>QGMDFTLNQEMLMTDTKSGALFYQEEEALSGVRKIANKVMHDVELVFGYQPEATKDRDMLSRHAVLYGTVGHSPLLDELNAAALIDLTEIAGKREVFLFQVVDQPIQGVEKALVIAGSDKRGTIYGLFHLSEKLGVSPLVDWSGVLPARKESFSLKGDYKYVSKEPSVKYRGFFINDEWPAFGNWSAKNFGGFNAEMYDHVFELLLRLKGNYLWPAMWSARFNDDGPGLANVELADEYGVIMGASHHEPCLRYGEEYKYLRGPDSIYGDAWNFITNREGITKFWEDGLKRTGHFENIITIGMRGEADTKIMGEDATLEDNINLLRDVIQTQNKLIKEHVNPNLKEVPRMLALYKEVEPFFYGDENTPGLINSEELEDVILMLCDDNHGNLRTLPTEDMRKHSGGYGMYYHFDYHGGPVSYEWINSSYLPKIWEQMTMAYDFGVRDLWIVNVGDIATQELPLSFFLDLAYDFDKWGTNAINKTDDYTKQWIEQQFAGVFNLEQKDKVFELLNGYTKIAHNRRPEAMNVDVYHPVNYHETDQLLDRIDHLLGLAEELYQEVDQQHFTAYFALVYYPTVGNLNLQKMWLLNGKNKYAAQLNLIEANKLAEQVKACLKRDQEIVDEYHTIADGKFYGMGLSEHIGFVHWNEDENKNPVLSYVLPVNKPRLLVSIDGTELRSEGSPWHVNTLPLVDFLEPDVNQASFTISSVSEKKAEYHISTDQDWLSCSAANGVLDGKNKLSETIHVFVDRDGLADQAEGRITVKTPVGKVTIVVPVVNNDFTNYPDMTFVDTKGYISIEAEHFATQKATENLDGTLNRFEV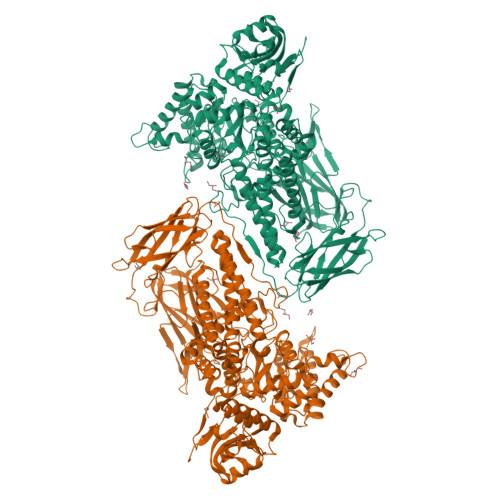LDGYGKTLSAIKAFPTDTHYQVGKDAPFVEYHFVTQEAGVYELEFYLQPSNPVTREGTMYAGIQVNENDVDVINVLPDGYHVDGPHWGIDVINNIRTTKTKITCEQGLNKLRIYAVSPGFALEKIVIYPDGKKLANSYLGPNETYYVGR[2x]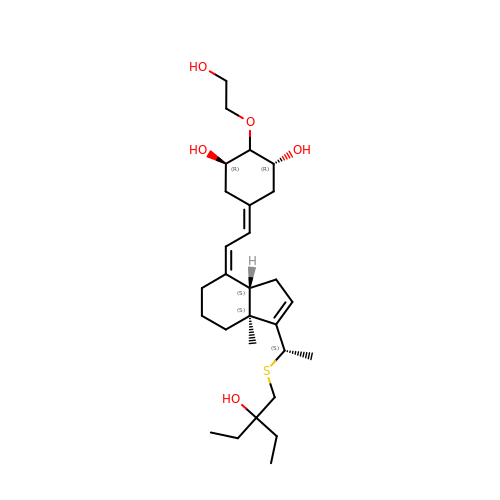(1R,2R,3R,5Z)-17-{(1S)-1-[(2-ethyl-2-hydroxybutyl)sulfanyl]ethyl}-2-(2-hydroxyethoxy)-9,10-secoestra-5,7,16-triene-1,3-diol | C28 H46 O5 S | DUIYWCMQVXJTIP-YYDWSLPPSA-N> MEEPEEPADSGQSLVPVYIYSPEYVSMCDSLAKIPKRASMVHSLIEAYALHKQMRIVKPKVASME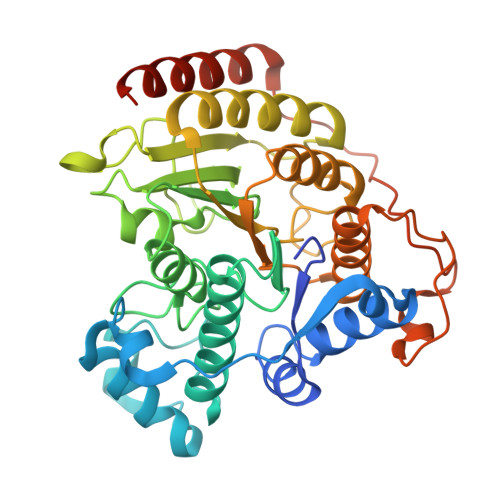EMATFHTDAYLQHLQKVSQEGDDDHPDSIEYGLGYDCPATEGIFDYAAAIGGATITAAQCLIDGMCKVAINWSGGWHHAKKDEASGFCYLNDAVLGILRLRRKFERILYVALDLHHGDGVEDAFSFTSKVMTVSLHKFSPGFFPGTGDVSDVGLGKGRYYSVNVPIQDGIQDEKYYQICESVLKEVYQAFNPKAVVLQLGADTIAGDPMCSFNMTPVGIGKCLKYILQWQLATLILGGGGFNLANTARCWTYLTGVILGKTLSSEIPDHEFFTAYGPDYVLEITPSCRPDRNEPHRIQQILNYIKGNLKHVVIEGRGSHHHHHH Among them, Cas12c2 binds a CRISPR RNA (crRNA) and a trans-activating crRNA (tracrRNA) and recognizes double-stranded DNA targets with a short TN PAM. Cas12c2 adopts a bilobed architecture consisting of recognition (REC) and nuclease (NUC) lobes. The REC lobe has the REC1, REC2, and PAM-interacting (PI) domains, and the NUC lobe comprises the WED and RuvC domains. Here, we present the cryo-electron microscopy (cryo-EM) structures of the Cas12c2–guide RNA binary complex and the Cas12c2–guide RNA–target DNA ternary complex, at overall resolutions of 3.0 Å and 2.7 Å, respectively.

To elucidate how Cas12c2 assembles with the sgRNA prior to the target DNA binding, we determined the cryo-EM structure of Cas12c2 in complex with the sgRNA at an overall resolution of 3.0 Å. In contrast, the Cas12c2–sgRNA binary complex adopts a closed conformation, in which the REC2 domain interacts with stem 3 of the tracrRNA. Notably, the PI domain is disordered in the binary complex structure, suggesting that the PI domain of Cas12c2 is flexible and stabilized by the interaction with the PAM duplex, whereas that of Cas12a is pre-ordered prior to DNA binding (Yamano et al., 2017). A structural comparison also revealed a local conformational change in the α1–α2 linker in the RuvC domain. In the binary complex, the α1–α2 linker adopts a loop conformation and interacts with the REC2 and WED domains, thereby stabilizing the closed conformation. The binary complex also revealed that only the first six nucleotides of the guide segment are ordered in the central channel, suggesting that nucleotides 1–6 in the guide segment serve as the important seed region for the R-loop formation, as in Cas12a (Swarts et al., 2017) and Cas12b (Yang et al., 2016). In the Cas12c2–sgRNA complex structure, the first six nucleotides within the 17-nucleotide spacer sequence are ordered, and the α1–α2 linker in the RuvC domain is located near the ordered sixth spacer nucleotide, suggesting that the linker region facilitates the bending of the pre-crRNA toward the RuvC active site for the processing reaction. In the Cas12c2 structure, the sixth nucleotide in the 17-nucleotide spacer sequence is blocked by the α1–α2 linker in the RuvC domain, and the rest of the spacer is disordered, suggesting that the pre-crRNA is kinked at this position and extends toward the RuvC active site for the pre-crRNA processing. In contrast, the corresponding region (residues 1014–1022) of Cas12c2 adopts similar loop conformations between the binary and ternary complexes, suggesting that the Lid motif is not involved in the RuvC domain activation in Cas12c2, as in Cas12a (Swarts et al., 2017).

> MKIEEGKGHHHHHHMTKHSIPLHAFRNSGADARKWKGRIALLAKRGKETMRTLQFPLEMSEPEAAAINTTPFAVAYNAIEGTGKGTLFDYWAKLHLAGFRFFPSGGAATIFRQQAVFEDASWNAAFCQQSGKDWPWLVPSKLYERFTKAPREVAKKDGSKKSIEFTQENVANESHVSLVGASITDKTPEDQKEFFLKMAGALAEKFDSWKSANEDRIVAMKVIDEFLKSEGLHLPSLENIAVKCSVETKPDNATVAWHDAPMSGVQNLAIGVFATCASRIDNIYDLNGGKLSKLIQESATTPNVTALSWLFGKGLEYFRTTDIDTIMQDFNIPASAKESIKPLVESAQAIPTMTVLGKKNYAPFRPNFGGKIDSWIANYASRLMLLNDILEQIEPGFELPQALLDNETLMSGIDMTGDELKELIEAVYAWVDAAKQGLATLLGRGGNVDDAVQTFEQFSAMMDTLNGTLNTISARYVRAVEMAGKDEARLEKLIECKFDIPKWCKSVPKLVGISGGLPKVEEEIKVMNAAFKDVRARMFVRFEEIAAYVASKGAGMDVYDALEKRELEQIKKLKSAVPERAHIQAYRAVLHRIGRAVQNCSEKTKQLFSSKVIEMGVFKNPSHLNNFIFNQKGAIYRSPFDRSRHAPYQLHADKLLKNDWLELLAEISATLMASESTEQMEDALRLERTRLQLQLSGLPDWEYPASLAKPDIEVEIQTALKMQLAKDTVTSDVLQRAFNLYSSVLSGLTFKLLRRSFSLKMRFSVADTTQLIYVPKVCDWAIPKQYLQAEGEIGIAARVVTESSPAKMVTEVEMKEPKALGHFMQQAPHDWYFDASLGGTQVAGRIVEKGKEVGKERKLVGYRMRGNSAYKTVLDKSLVGNTELSQCSMIIEIPYTQTVDADFRAQVQAGLPKVSINLPVKETITASNKDEQMLFDRFVAIDLGERGLGYAVFDAKTLELQESGHRPIKAITNLLNRTHHYEQRPNQRQKFQAKFNVNLSELRENTVGDVCHQINRICAYYNAFPVLEYMVPDRLDKQLKSVYESVTNRYIWSSTDAHKSARVQFWLGGETWEHPYLKSAKDKKPLVLSPGRGASGKGTSQTCSCCGRNPFDLIKDMKPRAKIAVVDGKAKLENSELKLFERNLESKDDMLARRHRNERAGMEQPLTPGNYTVDEIKALLRANLRRAPKNRRTKDTTVSEYHCVFSDCGKTMHADENAAVNIGGKFIADIEK>[2x]MKHLHRFFSSDASGGIILIIAAILAMIMANSGATSGWYHDFLETPVQLRVGSLEINKNMLLWINDALMAVFFLLVGLEVKRELMQGSLASLRQAAFPVIAAIGGMIVPALLYLAFNYADPITREGWAIPAATDIAFALGVLA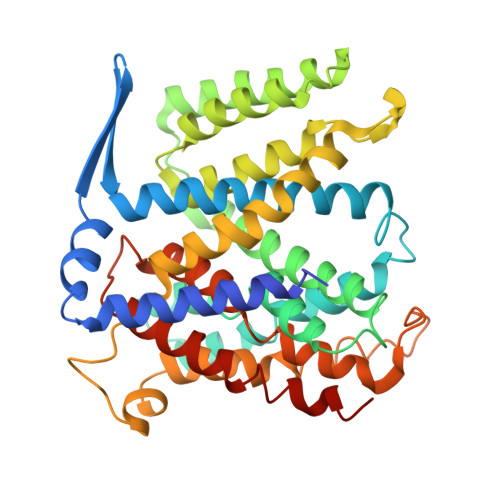LLGSRVPLALKIFLMALAIIDDLGAIIIIALFYTNDLSMASLGVAAVAIAVLAVLNLCGARRTGVYILVGVVLWTAVLKSGVHATLAGVIVGFFIPLKEKHGRSPAKRLEHVLHPWVAYLILPLFAFANAGVSLQGVTLDGLTSILPLGIIAGLLIGKPLGISLFCWLALRLKLAHLPEGTTYQQIMVVGILCGIGFTMSIFIASLAFGSVDPELINWAKLGILVGSISSAVIGYSWLRVRLRPSV IMP-13, a member of subgroup 2, sharing 92.3% amino acid sequence similarity with IMP-2 and 82.5% with IMP-1 (Fig. SI2), was first identified in the Gram-negative pathogen Pseudomonas aeruginosa from clinical samples in Italy and is a common cause of carbapenem resistance, often involved in large outbreaks. Imipenemases represent one of the major groups of class B1 metallo-β-lactamases found in Gram-negative pathogens, and these enzymes can hydrolyze all bicyclic β-lactam antibiotics. The overall protein architecture of the IMP-13 apo structure is consistent with that of the previously published metallo-β-lactamase fold, consisting of a global αβ/βα topology with a shallow active-site cleft at the border of the two β-sheets. The structural information and dynamics presented here reveal important information about the mechanism of antibiotic binding, as well as a significant role for the active-site-covering loop (L1), indicating that the plasticity of the active-site region is important for the broad substrate recognition spectrum of these enzymes.

In the apo-state crystal structures, two positions for the L1 loop, open and closed, were observed. The L1 loop adopts very different conformations in the two apo structures (apoclosed and apoopen). In the apoclosed structure, the loop is folded over the active site, while in the apoopen structure, L1 is extended away from the protein, leaving the active site accessible. We define the open conformation to be the loop pointing away from the protein toward the solvent and the closed conformation to be the loop positioned over the active site and pointing toward its rim. The distance between C-α atoms of Trp28 for the open and closed conformations is 8.8 Å. With the apoopen structure, on the other hand, the loop can be seen to point away from the active site, leaving the active site accessible to the substrate. The tunnel formation seen in the closed form is completely absent due to the different positioning of both backbone and side chain atoms. On the other hand, the ability of the loop to adopt a fully open state, as observed in the apoopen structure of IMP-13, provides an alternative strategy for inhibitor development. As the loop appears to play an active role in the binding of ligands to the protein, prevention of the loop closing by an allosteric inhibitor could have a similar inhibitory effect.

>LPDLKIEKLEEGVFVHTSFEEVNGWGVVTKHGLVVLVNTDAYLIDTPFTATDTEKLVNWFVERGYEIKGTISSHFHSDSTGGIEWLNSQSIPTYASELTNELLKKSGKVQAKYSFSEVSYWLVKNKIEVFYPGPGHTQDNLVVWLPESKILFGGCFIKPHGLGNLGDANLEAWPKSAKILMSKYGKAKLVVSSHSEKGDASLMKRTWEQALKGLKESKKT[4x]>MTETPATPTGLPTARAAGCPFDPPPGLAALRDRAPLTRMEFPNGHVGWLATGHAVVRAVLADPRFSHRNDRRHWPLADIGRGFPPLPGDMLHIDPPDHTRYRKLLAGKFTMRRMRRLTGSAQEIVAGKLDAMERHGGPLDLLEFFARPVPTLMVCALLGVPLQDRATFHPPVRGTDDAAAVEADVAAYVEMTYADMQEYFRKLVAAKRAAPADDLLSDLTTSDLTEDELVGLCAVMMHAGVDSTSNMLALGTWALLERPDQLAALRERPDLADRAVEELMRYMSVVHTGSRAALEDVELAGEVVRAGESVAFSVQAANRDPARFADPDTLDI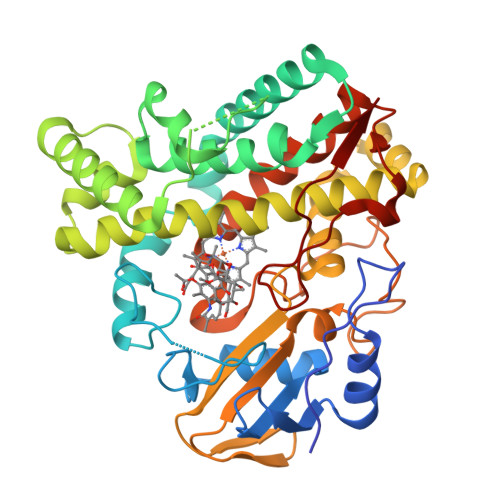RRGAVGHLGFGYGVHQCLGMQLARVEMRVAFPALFARFPALRLAVPAGDVPMRDDLVIPYGVHRLPVTW[2x]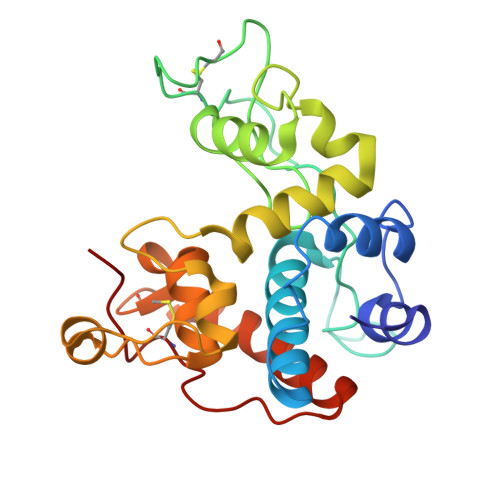> MVSRSMFDQLFKHRNSFYTYDAFIAAAKSFPSFGTTGDTDVRKREIAAFFAHVSHETTGGWPTAPDGPYAWGLVYIEEINQSNDYCDPSTQYPCAPGKQYYGRGPLQLSWNYNYGPCGDALGLDLLNNPDLVAQDPVIAFKTALWFWMTPQSPKPSCHDVMTGNWTPSSADLAAGRVPGFGVTTNIINGGLECGKGNPAQAENRVGFYKRFCNQLGVSPGSNLDCANMRPFG> MGSSHHHHHHSSGRENLYFQGHMNGDQNSDVYAQEKQDFVQHFSQIVRVLTEDEMGHPEIGDAIA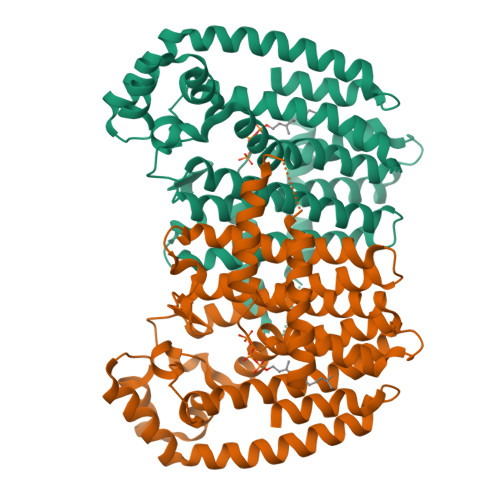RLKEVLEYNAIGGKYNRGLTVVVAFRELVEPRKQDADSLQRAWTVGWCVELLQAFFLVADDIMDSSLTRRGQICWYQKPGVGLDAINDANLLEACIYRLLKLYCREQPYYLNLIELFLQSSYQTEIGQTLDLLTAPQGNVDLVRFTEKRYKSIVKYKTAFYSFYLPIAAAMYMAGIDGEKEHANAKKILLEMGEFFQIQDDYLDLFGDPSVTGKIGTDIQDNKCSWLVVQCLQRATPEQYQILKENYGQKEAEKVARVKALYEELDLPAVFLQYEEDSYSHIMALIEQYAAPLPPAVFLGLARKIYKRRK> MATSRYEPVAEIGVGAYGTVYKARDPHSGHFVALKSVRVPNGEEGLPISTVREVALLRRLEAFEHPNVVRLMDVCATSRTDREIKVTLVFEHVDQDLRTYLDKAPPPGLPAETIKDLMRQFLRGLDFLHANCIVHRDLKPENILVTSGGTVKLADFGLARIYSYQMALAPVVVTLWYRAPEVLLQST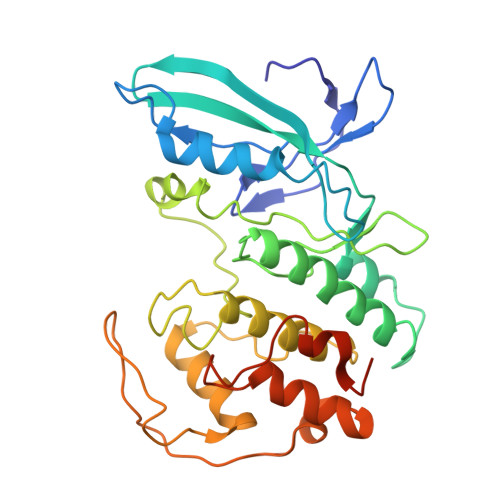YATPVDMWSVGCIFAEMFRRKPLFCGNSEADQLGKIFDLIGLPPEDDWPRDVSLPRGAFPPRGPRPVQSVVPEMEESGAQLLLEMLTFNPHKRISAFRALQHSYLHKDEGNPEHHHHHH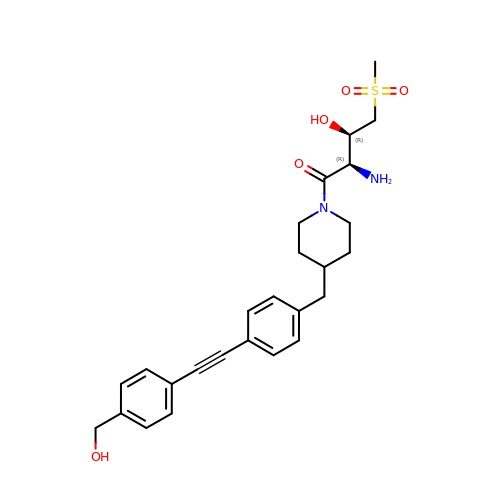(2R,3R)-2-azanyl-1-[4-[[4-[2-[4-(hydroxymethyl)phenyl]ethynyl]phenyl]methyl]piperidin-1-yl]-4-methylsulfonyl-3-oxidanyl-butan-1-one | C26 H32 N2 O5 S | RNBZGRMVKCFVJP-LOSJGSFVSA-N>[2x]ASMPAVERQLIECLHHVIKGAEPQQVGILCPQDDQRKALTEQFGSKTATSFCKEVDSLKNLSNLDALIVNQALDEEINDSEKLDKFITAALRSLRTDGVLILRQDLSKVKEMKKMAMLTDYFDVFRLEEGNGNVGFQFYAVNEVLDSVYVHQNWLDFI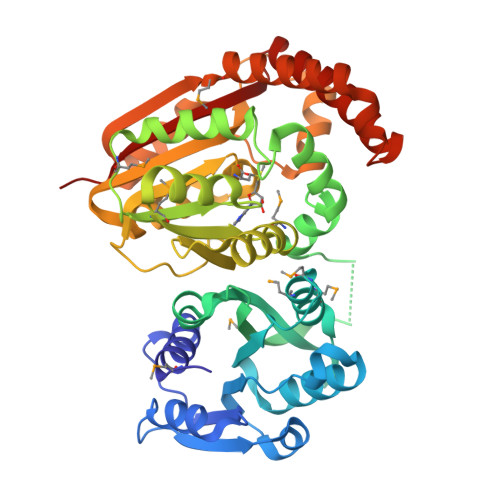WTLMKKPFPKDINGVVSFRDFLDRTQYTDTGIFAYEWIFGNNFISPGGWNQNLAILKRFGPMKTGQRMLDIGVGIGGGARQAASEFGLQVHGVDLSTNMLAVALERVHKEKDARVTYAVCDACEYEFEPNSFDYVFSRDCIQHIKDTDKLFSRIYRALKPGGKVLITMYGVGHGTLSESFKEYVSQRQYYLKNLEQIEEIAKKTGFIDIEVENMTPRFKEILLEERERIEQDKETFLAKFSQNAYDGLVSGWKSKLQYIADDNHNWNFFAAVKPQ>[2x]MNIIGFSKALFSTWIYYSPERILFDAGEGVSTTLGSKVYAFKYVFLTHGHVDHIAGLWGVVNIRNNGMG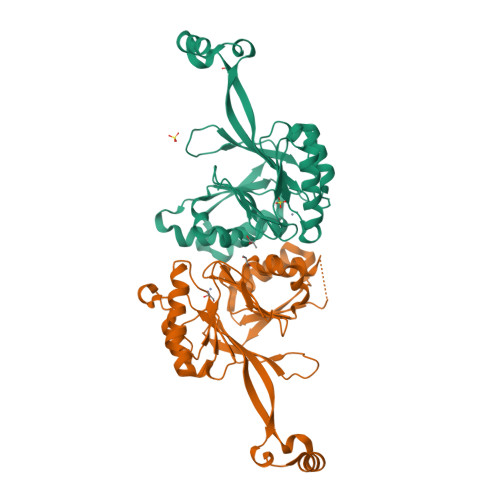DREKPLDVFYPEGNRAVEEYTEFIKRANPDLRFSFNVHPLKEGERVFLRNAGGFKRYVQPFRTKHVSSEVSFGYHIFEVRRKLKKEFQGLDSKEISRLVKEKGRDFVTEEYHKKVLTISGDSLALDPEEIRGTELLIHECTFLDARDRRYKNHAAIDEVMESVKAAGVKKVILYHISTRYIRQLKSVIKKYREEMPDVEILYMDPRKVFEM> MATKEQIVEHRESEIPIASQWKATFPVDLEIEKNSEMFALRYIKCASAFILDRRGILDEKCFKTRTIDKLLVTAFQSSVPAAKRVSSTFDGLYDAIQQGYLREFAIVFYKKPNEEDINEVFAFRFAYGDEGEIFVSLNNGIDTNESSQELLQAKFVDTDNTKQMFASTIKKLHRCIKKMEPLPQGSDASFRVSYTEKAPKDYTPEGYLLSPMFYTLNQDIRKASIGIVCGGHHKIQMLAASQYLKQDF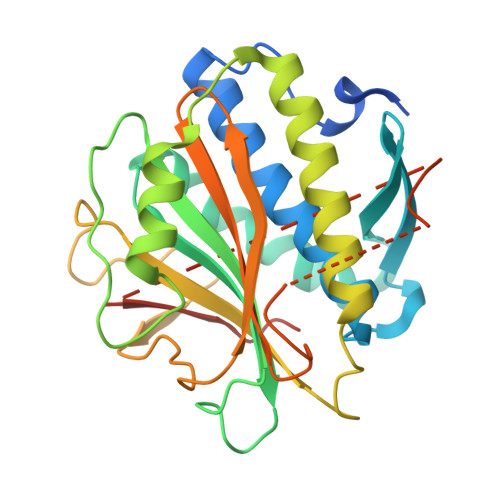DLDKTTTLNPNMSIMANQSKRKGRISRDSPYGLSQGITKKNKD heptyl 3-fluoro-alpha-D-mannopyranoside | 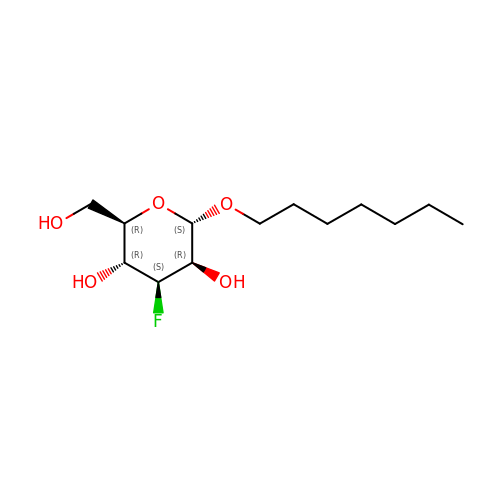C13 H25 F O5 | ZEXHYSKAVKHNNT-FHUSYTEZSA-N>[2x]GPGSELPQMVQQLNSPDQQELQSALRKLSQIASGGDEQIQAVIDAGALPALVQLLSSPNEQILQEALWTLGNIASGGDEQIQAVIDAGALPALVQLLSSPNEQILQEALWTLGNIASGGDEQIQAVIDAGAL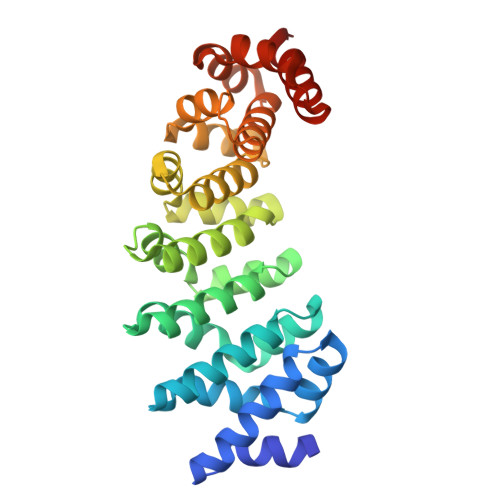PALVQLLSSPNEQILQEALWTLGNIASGGDEQIQAVIDAGALPALVQLLSSPNEQILQEALWTLGNIASGGDEQIQAVIDAGALPALVQLLSSPNEQILQEALWTLGNIASGGNEQKQAVKEAGALEKLEQLQSHENEKIQKEAQEALEKLQSH>MKLSDLISRWIDVEPSKNAQIILRDRYFMKDLDGNYLETKWEDVARRVARVVATAELLNPSYKKNEKLDRIKEWEDIFFRVLKARLFIPNSPTLFNAGLGVKHDLLWKPIDQMTLEDYEEIYRSRNHLHMLSACFVVPVGDSIEEIFEAVKEYALITKVGGGVGSNFSELRPKGSFVAGTHGKASGPVSFMHVFNSAISVVKQGSRRRGALMGILNINHPDIEEFIDAKKENTGEAVLNF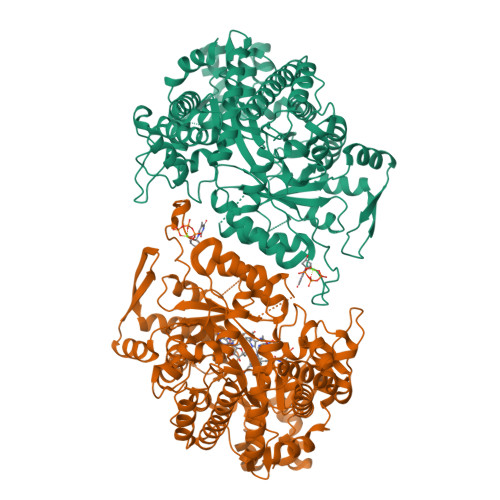FNLSVGFPMDKKEILKLYEEDGELELSHPRSTIRKKVKIRELFRKIATNAWKSGDPGLAFLGEMNKYYPLYPHRKINSTNPCGEIGLSDYEACNLGSIDVAKFYNNGFVDLEALQELVQIAVRFLDNVIDVNVFPIDKITKAVKESRRLGLGIMGFADLLYKLEIPYNSQEARDFAANLMAFIALHAHRTSYELGKEKGNFPLLEISRYRTEDNFVPFAMGMSNYDDEIREVMKMTKEFRRNVALLTIAPTGSISNIADTSSGLEPNFLLAYTRFVTKEDGTKEPLLYVNQVLREKLNPEILKRIEKELIEKGSLKDIPDVPEKIKKVFVVALDIDPMDHLLMQDAFQRYVDNNISKTINMPQSATVDDVLNVYLEALRTNVRGITVYRDGSLQTQVLTKALKT[2x]>[2x]GHHHHHHHHHHSSGHIEGRHMKPSFSPRNYKALSEVQGWKQRMAAKELARQNMDLGFKLLKKLAFYNPGRNIFLSPLSISTAFSMLCLGAQDSTLDEIKQGFNFRKMPEKDLHEGFHYIIHELTQKTQDLKLSIGNTLFIDQRLQPQRKFLEDAKNFYSAETILTNFQNLEMAQKQINDFISQKTHGKINNLIENIDPGTVMLLANYIFFRARWKHEFDPNVTKEEDFFLEKNSSVKVPMMFRSGIYQVGYDDKLSCTILEIPYQKNITAIFILPDEGKLKHLEKGLQVDTFSRWKTLLSRRVVDVSVPRLHMTGTFDLKKTLSYIGVSKIFEEHGDLTKIAPHRSLKVGEAVHKAELKMDERGTEGAAGTGAQTLPMETPLVVKIDKPYLLLIYSEKIPSVLFLGKIVNPIGK

Previously, visceral adipose tissue-derived serpin (referred to as vaspin in this paper; serpinA12 according to the serpin nomenclature) was identified as a putative member of the serine protease inhibitor family, which was expressed in visceral adipose tissue of Otsuka Long-Evans Tokushima Fatty (OLETF) rats at the age when obesity and insulin plasma concentrations reach a peak. Here, we provide the vaspin crystal structure and identify human kallikrein 7 (hK7) as a first protease target of vaspin inhibited by classical serpin mechanism with high specificity in vitro. We provide evidence that the serpin function of vaspin is essential for its physiologic effects and demonstrate that the anti-diabetic vaspin effects in vivo do not result from increased insulin sensitivity but are rather based on an insulin-stabilizing effect most likely by inhibiting hK7-mediated insulin degradation.

Based on sequence homology with α1-antitrypsin vaspin has been predicted to belong to the serpin protein family. After expression, purification and crystallization of recombinant human vaspin, X-ray structure determination confirmed the typical structural core domains of serpins consisting of three β-sheets and nine α-helices. As expected, nearby regions match closely in a superposition onto related serpins. The fold corresponds to that of free serpins or serpins involved in a transient complex, i.e. the long central β-sheet consists of five strands. The reactive center loop (RCL) (extending from G364 to P381) is flexible in the vaspin structure. The P15 glycine is located in a tight turn between anti parallel β-strands and is highly conserved within the serpin family, most likely because torsion angles in this conformation are only allowable for the least restricted amino acid glycine in the Ramachandran plot. It has been shown that the serpin inhibitory mechanism is critically dependent on the length of the RCL and is furthermore structurally based on conserved small side-chain amino acids within the hinge region of inhibitory serpins. The variant vaspinA369P fails to inhibit hK7 activity and the mutation prevents complex formation with the protease. Comparison of the RCL sequences of vaspin and other prominent serpins suggested methionine 378 as P1 residue, though tyrosine is the preferred P1 residue. Indeed, we could confirm methionine 378 as P1 residue for hK7 in vaspin by mass spectrometry.>[4x]HHHHHHSSGLV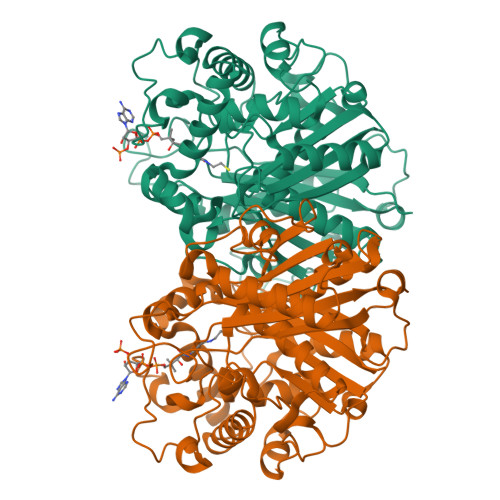PRGSHMFRSSLTHLQAASRVFIVGGHITPFVGKGSPLFIDKKHPDFGKKKNMTLEEILATTVQGTMEHSGLSGREGIVDQVVVGNFLGELFSSQGHLGPAAIGSLTYGQAGSKNPLMYKPAMRVEGAAASGGLAVISAMNALKSGSADITLAVGVEVQTTASARVGGDYLARAADYQRQRQLDDFTFPCLFAKRMKYIAEHNHFTMEDTARVAAKAYANGNKNPLAHMHTRKLTFEQCNGEDPSNVKFLGNETYKEYLRMTDCSQVSDGGAGVVLANEEGLRKMGLSPNDSRLVEIKSIACAVSNLYEDPDDACCMFTSRQAAQKALSMANIKPSDLNVAEVHDCFTIAEMLMYEALGIAEYGHAKDLIRNGDTTLEGRIPVNTGGGLLSFGHPVGATGIKQIMEVYRQMKGQCEAYQMKKIPALGATLNMGGDDKTAVSAVLQNI>MKIGVFDSGVGGFSVLKSLLKARLFDEIIYYGDSARVPYGTKDPTTIKQFGLEALDFFKPHEIELLIVACNTASALALEEMQKYSKIPIVGVIEPSILAIKRQVEDKNAPILVLGTKATIQSNAYDNALKQQGYLNISHLATSLFVPLIEESILEGEL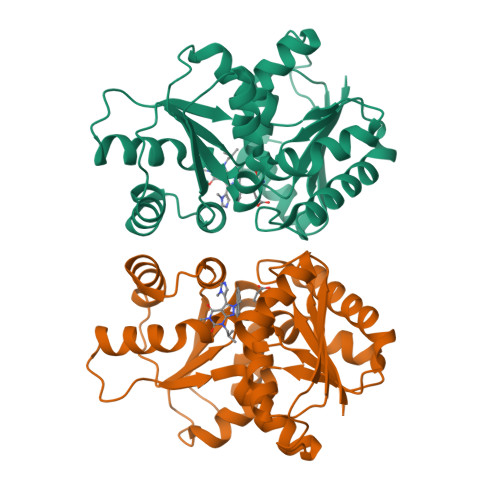LETCMHYYFTPLEILPEVIILGCTHFPLIAQKIEGYFMGHFALPTPPLLIHSGDAIVEYLQQKYALKNNACTFPKVEFHASGDVIWLERQAKEWLKL[2x]> VTSVEQRTATAVFSRTGSRMAERRLAFMLVAPAAMLMVAVTAYPIGYALWLSLQRNNLATPNDTAFIGLGNYHTILIDRYWWTALAVTLAITAVSVTIEFVLGLALALVMHRTLIGKGLVRTAVLIPYGIVTVVASYSWYYAWTPGTGYLANLLPYDSAPLTQQIPSLGIVVIAEVWKTTPFMSLLLLAGLALVPEDLLRAAQVDGASAWRRLTKVILPMIKPAIVVALLFRTLDAFRIFDN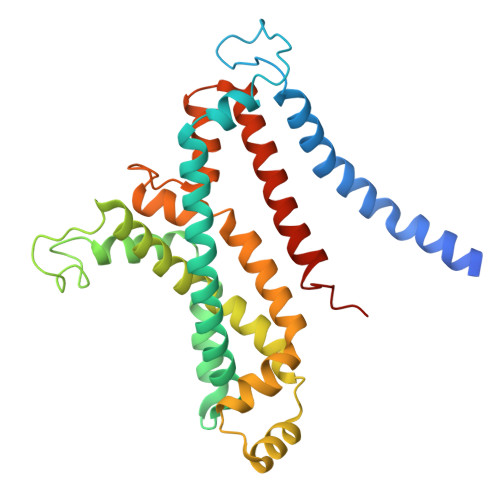IYVLTGGSNNTGSVSILGYDNLFKGFNVGLGSAISVLIFGCVAVIAFIFIKLFGAAAPGGEPSGR> MKTADLCDQFLDELQVCELPFQSYGGKRMFSGPIATVDVFEDNVLVREALETVPPGTVLVVDGKGSRR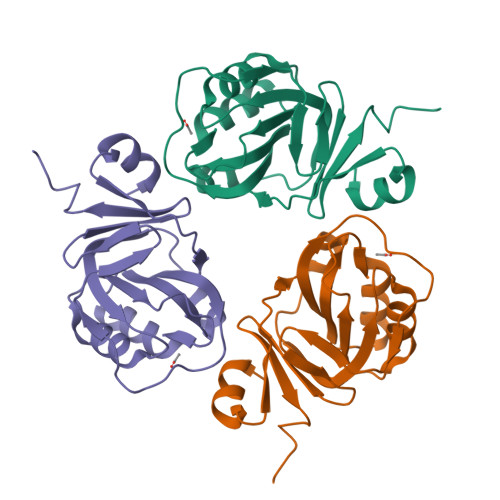VALLGDRLAQIACERGLAGVIIHGCIRDSAEIGAMPIGVMAIGTCPVKSKKEGKGARDVVLEFGGVRWEPGAYVYADADGVVVANKDLLAKNG>[2x]QTQVLFEHP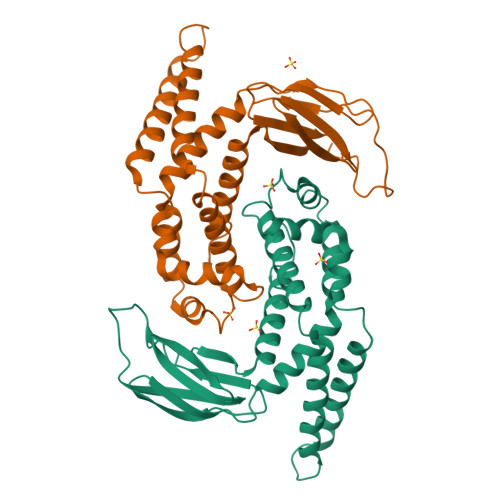LNEKMRTWLRIEFLIQQLTVNLPIVDHAGALHFFRNVSELLDVFERGEVRTELLKELDRQQRKLQTWIGVPGVDQSRIEALIQQLKAAGSVLISAPRIGQFLREDRLIALVRQRLSIPGGCCSFDLPTLHIWLHLPQAQRDSQVETWIASLNPLTQALTMVLDLIRQSAPFRKQTSLNGFYQDNGGDADLLRLNLSLDSQLYPQISGHKSRFAIRFMPLDTENGQVPERLDFELACC> GSVDIEVQDLEEFALRPAPQGITIKCRITRDKKGMD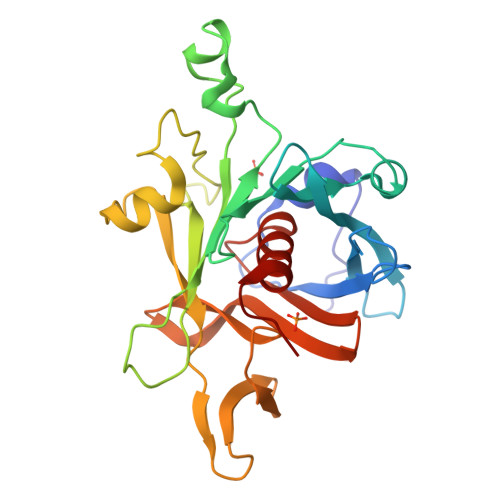RGMFPTYFLHLDREDGKKVFLLAGRKRKKSKTSNYLISVDPTDLSRGGDSYIGKLRSNLMGTKFTVYDNGVNPQKASSSTLESGTLRQELAAVCYETNVLGFKGPRKMSVIVPGMNMVHERVCIRPRNEHETLLARWQNKNTESIIELQNKTPVWNDDTQSYVLNFHGRVTQASVKNFQIIHGNDPDYIVMQFGRVAEDVFTMDYNYPLCALQAFAIALSSFDSKLACE5-[4-bromo-2-(2-chloro-6-fluorophenyl)-1H-imidazol-5-yl]-2-{[4-(trifluoromethyl)phenyl]ethynyl}pyridine 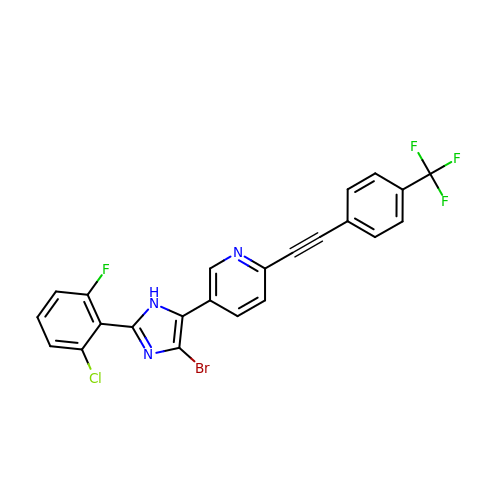| C23 H11 Br Cl F4 N3 | KPXLXMUZOLULFL-UHFFFAOYSA-N> MRLFVSDGVPGCLPVLAAAGRARGRAEVLISTVGPQDCVVPFLTRPKVPVLQLDSGNYLFSTSAICRYFFLLSGWEQDDLTNQWLEWEATELQPALSAALYYLVVQGKKGEDVLGSVRRALTHIDHSLSRQNCPFLAGETESLADIVLWGALYPLLQDPAYLPEELSALHSWFQTLSTQEPCQRAAQTVLKQQGVLALRPYLQKQPQLEHHHHHH;> GHMAAAAELSLLEKSLGLSKGNKYSAQGERQIPVLQTNDGPSLMGLTTIAAHLVKQANKEYLLGSTAEEKAMVQQWLEYRVTQVDGHSSKNDIHTLLMDLNSYLEDKVYLTGYNFTLADILLYYGLHRFIVDLTVQEKEKYLN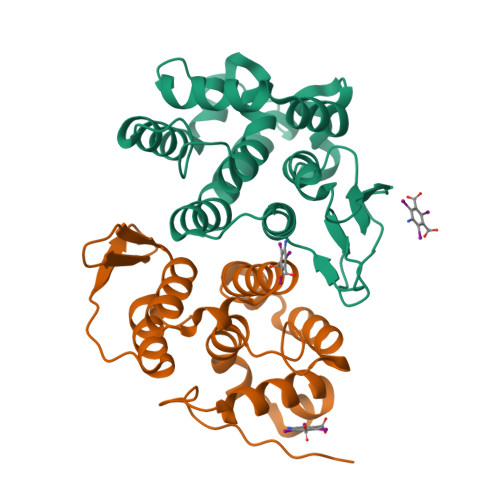VSRWFCHIQHYPGIRQHLSSVVFIKNRL>[2x]GSNRRLQQTQAQVDEVVDIMRVNVDKVLERDQKLSELDDRADALQAGASQFETSAAKLKRKYW;>[2x]ALSEIETRHSEIIKLENSIRELHDMFMDMAMLVESQGEMIDRIEYNVEHAVDYVERAVSDTKKAVK;>[2x]NELEEMQRRADQLADESLESTRRMLQLVEESKDAGIRTLVMLDEQGEQLDRVEEGMNHINQDMKEAEKNLKDLGK;>ARENEMDENLEQVSGIIGNLRHMALDMGN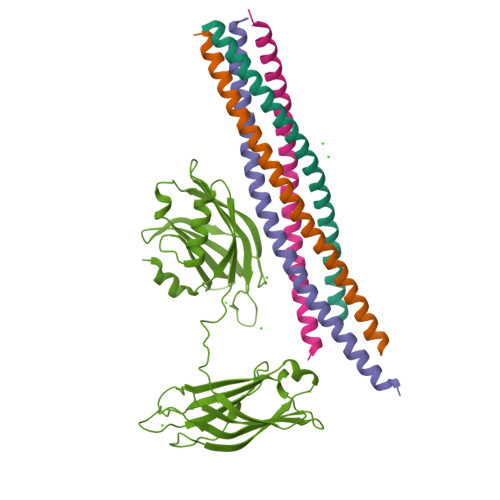EIDTQNRQIDRIMEKADSNKTRIDEANQRATKMLG[2x];>[3x]KLGKLQYSLDYDFQNNQLLVGIIQAAELPALDMGGTSDPYVKVFLLPDKKKKFETKVHRKTLNPVFNEQFTFKVPYSELGGKTLVMAVYDFDRFSKHDIIGEFKVPMNTVDFGHVTEEWRDLQSAEKEEQEKLGDICFSLRYVPTAGKLTVVILEAKNLKKMDVGGLSDPYVKIHLMQNGKRLKKKKTTIKKNTLNPYYNESFSFEVPFEQIQKVQVVVTVLDYDKIGKNDAIGKVFVGYNSTGAELRHWSDMLANPRRPIAQWHTLQVEEEVDAMLAV>[3x]ASNFEEFVLVDNGGTGDVKVAPSNFANGVAEWISSNSRSQAYKVTCSVRQSSANNRKYTVKVEVPKVATGVELPVAAWR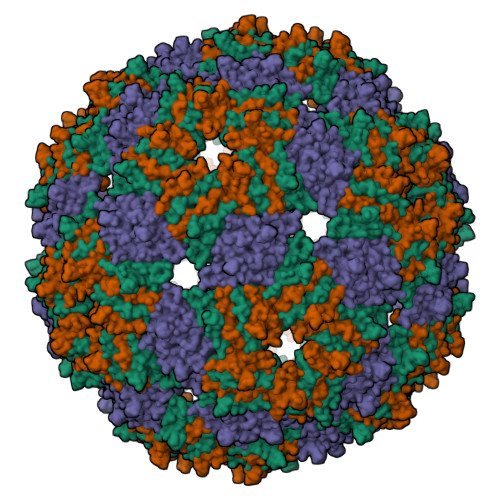SYMNMELTIPVFATNDDCALIVKALQGTFKTGNPIATAIAANSGIY4-BROMO-L-PHENYLALANINE | C9 H10 Br N 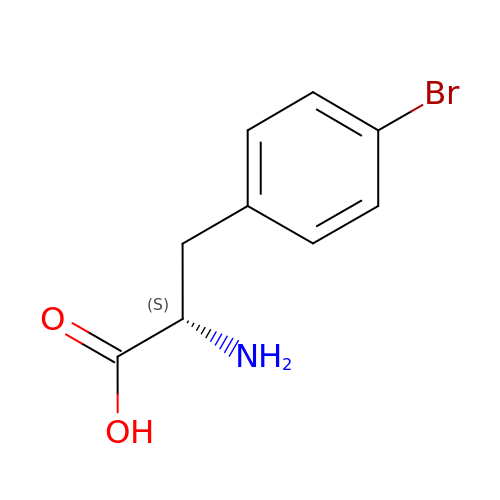O2 | PEMUHKUIQHFMTH-QMMMGPOBSA-N TatD is a conserved protein widely expressed in different species, including bacteria, fungi, plants and animals. Here we provide lines of evidence showing that TatD is a 3′–5′ exonuclease that processes single-stranded DNA in DNA repair. TatD represents the first example of a TIM-barrel exonuclease that hydrolyzes the phosphodiester bond at the 3′ end of a nucleic acid chain. TatD has a TIM-barrel fold and it trims DNA from 3′-to-5′ ends in the hydrogen peroxide-induced DNA repair, including double-strand break repair and nucleotide excision repair in E. coli.

To understand how TatD binds and cleaves DNA, we further co-crystallized TatD with a single-stranded DNA (5′-GCTTAGCT-3′). TatD–DNA complex was crystallized by the hanging-drop vapor diffusion method and the co-crystal diffracted X-ray to a resolution of 2.9 Å. The simulated annealing omit Fourier map (2Fo − Fc) of the bound DNA revealed weak electron density for the three nucleotides (5′-G-p-C-p-T-3′). The 8-nucleotide single-stranded DNA was likely digested by TatD and resulted a 3-nucleotide DNA. Alternatively, it is possible that the 5′ end of the DNA was disordered and only the three nucleotides at the 3′ end were observed. The DNA was refined with an occupancy of 0.7 and an averaged B-factor of 69.2 Å2 and was bound at the loop region on the top of the TIM-barrel in a way similar to that of Endo IV. Superimposition of the apo-form and DNA-bound TatD gave an average RMSD of 0.394 Å for 259 Cα atoms, suggesting that DNA binding did not induce any major conformational change. However, a close look at the protein–DNA interface showed that the loop with R98 and F100 moved toward DNA in the TatD–DNA complex structure, and as a result, the two residues, R98 and F100 were disordered and refined with an occupancy of 0.79 and 0.85, respectively. Moreover, the residue H64 near the scissile phosphate had two alternative conformations and was refined with an occupancy of 0.53 (apo-form conformation) and 0.47 (flip-out conformation), respectively. However, no metal ion was identified in the TatD–DNA complex structure and DNA is bound loosely between two TatD molecules in the crystal, indicating that the 5′-G-p-C-p-T-3′ was bound in an inactive conformation.

> MFDIGVNLTSSQFAKDRDDVVACAFDAGVNGLLITGTNLRESQQAQKLARQYSSCWSTAGVHPHDSSQWQAATEEAIIELAAQPEVVAIGECGLDFNRNFSTPEEQERAFVAQLRIAADLNMPVFMHCRDAHERFMTLLEPWLDKLPGAVLHCFTGTREEMQACVAHGIYIGITGWVCDERRGLELRELLPLIPAEKLLIETDAPYLLPRDLTPKPSSRRNEPAHLPHILQRIAHWRGEDAAWLAATTDANVKTLFGIAF>MEFKDFPLKPEILEALHGRGLTTPTPIQAAALPLALEGKDLIGQARTGTGKTLAFALPIAERLAPSQERGRKPRALVLTPTRELALQVASELTAVAPHLKVVAVYGGTGYGKQKEALLRGADAVVATPGRALDYLRQG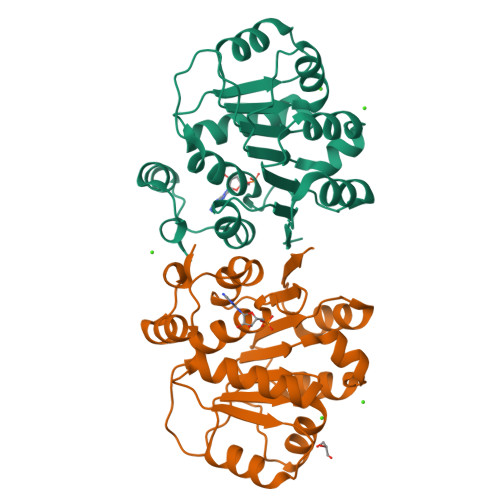VLDLSRVEVAVLDEADEMLSMGFEEEVEALLSATPPSRQTLLFSATLPSWAKRLAERYMKNPVLINVIK[2x]> GSPEFRSMTAIEDILQITTDPSDTRGYSLLKSEEVPQGSTLGVDFIDTLLLYQLTENEKLDKPFEYLNDCFRRNQQQKRITKNKPNAESLHSTFQEIDRLVIGYGVVALQIENFCMNGAFINYITGIVSNVNSYTDFLSQIIQRAILEGTALDLLNAVFPTLLEYCNKHVSHFDLNESVIYNNVLTIFELFVTFKPIAEIFTKIDGFFADYSCKPQDFERKTILGPILSLSPIEAAVAIRNYGDNLLRSKQQTAMIHESLQAEHKVVIDRLFFIVDKLVRGSLNSRTDMISYFAHIANKNHLRRADHPPFKELSSNGFMSNITLLLVRFSQPFLDISYKKIDKIDANYFNNPSLFIDLSGETRLNSDFKEADAFYDKNRKTADSKPNFISDCFFLTLTYLHYGLGGTLSFEEKMGSEIKALKEEIEKVKKIAANHDVFARFITAQLSKMEKALKTTESLRFALQGFFAHRSLQLEVFDFICGASTFLIRVVDPEHEFPFKQIKLPLIPDQIGVENVDNADFLRAHAPVPFKYYPEFVVEGPV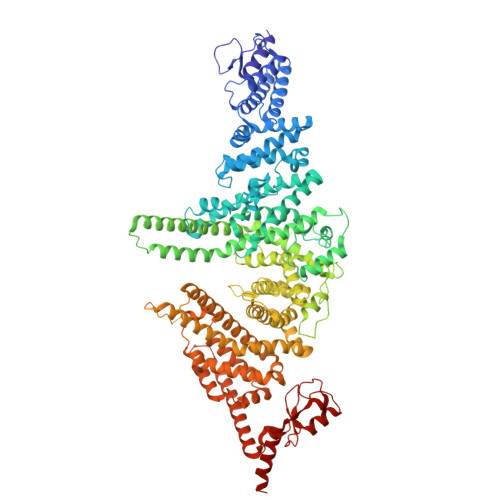NYSLYISKYQTSPIFRNPRLGSFVEFTTMVLRCPELVSNPHLKGKLVQLLSVGAMPLTDNSPGFMMDIFEHDELVNKNLLYALLDFYVIVEKTGSSSQFYDKFNSRYSISIILEELYYKIPSYKNQLIWQSQNNADFFVRFVARMLNDLTFLLDEGLSNLAEVHNIQNELDNRARGAPPTREEEDKELQTRLASASRQAKSSCGLADKSMKLFEIYSKDIPAAFVTPEIVYRLASMLNYNLESLVGPKCGELKVKDPQSYSFNPKDLLKALTTVYINLSEQSEFISAVAKDERSFNRNLFVRAVDILGRKTGLASPEFIEKLLNFANKAEEQRKADEEEDLEYGDVPDEFLDPLMYTIMKDPVILPASKMNIDRSTIKAHLLSDSTDPFNRMPLKLEDVTPNEELRQKILCFKKQKKEEAKHKASE Flurazepam | C21 H23 Cl F N3 O | 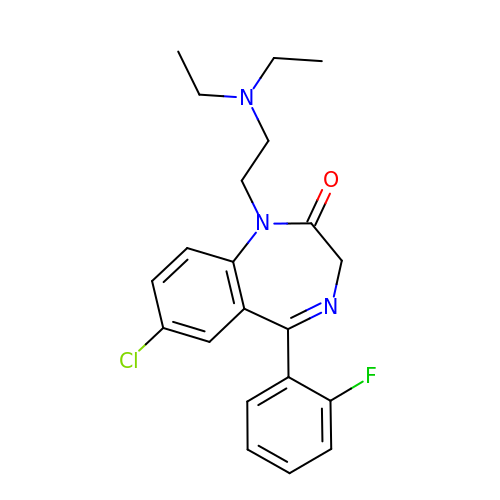SAADBVWGJQAEFS-UHFFFAOYSA-N2-ETHOXYETHYLPHOSPHINATE | C4 H10 O3 P | 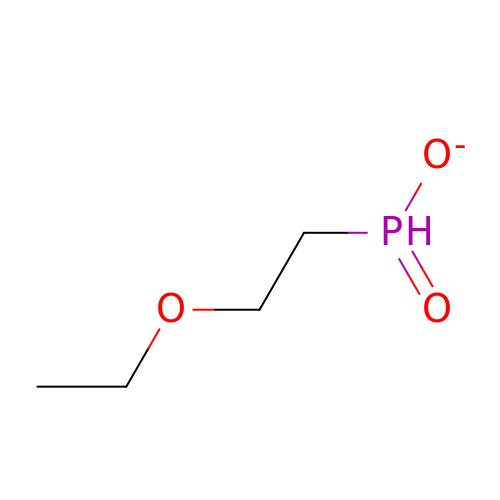XCMXNBBWZYFHSD-UHFFFAOYSA-M> MHHHHHHAAGIPMNNPAIKRIGNHITKSPEDKREYRGLELANGIKVLLISDPTTDKSSAALDVHIGSLSDPPNIAGLSHFLQHMLFLGTKKYPKENEYSQFLSEHAGSSNAFTSGEHTNYYFDVSHEHLEGALDRFAQFFLSPLFDESAKDREVNAVDSEHEKNVMNDAWRLFQLEKATGNPKHPFSKFGTGNKYTLETRPNQEGIDVRQE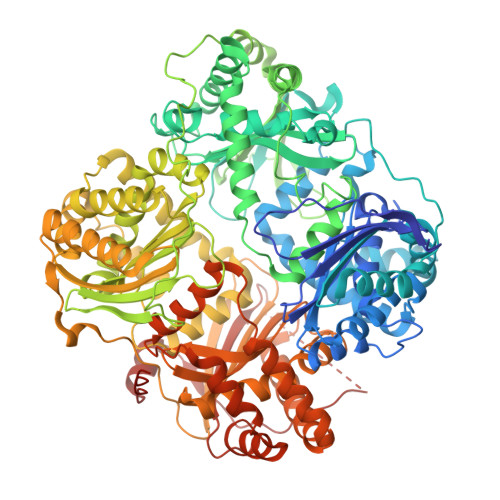LLKFHSAYYSSNLMAVVVLGRESLDDLTNLVVKLFSEVENKNVPLPEFPEHPFQEEHLKQLYKIVPIKDIRNLYVTFPIPDLQKYYKSNPGHYLGHLIGHEGPGSLLSELKSKGWVNTLVGGQKEGARGFMFFIINVDLTEEGLLHVEDIILHMFQYIQKLRAEGPQEWVFQELKDLNAVAFRFKDKERPRGYTSKIAGILHYYPLEEVLTAEYLLEEFRPDLIEMVLDKLRPENVRVAIVSKSFEGKTDRTEEWYGTQYKQEAIPDEVIKKWQNADLNGKFKLPTKNEFIPTNFEILPLEKEATPYPALIKDTAMSKLWFKQDDKFFLPKANLNFEFFSPFAYVDPLHSNMAYLYLELLKDSLNEYAYAAELAGLSYDLQNTIYGMYLSVKGYNDKQPILLKKIIEKMATFEIDEKRFEIIKEAYMRSLNNFRAEQPHQHAMYYLRLLMTEVAWTKDELKEALDDVTLPRLKAFIPQLLSRLHIEALLHGNITKQAALGIMQMVEDTLIEHAHTKPLLPSQLVRYREVQLPDRGWFVYQQRNEVHNNSGIEIYYQTDMQSTSENMFLELFAQIISEPAFNTLRTKEQLGYIVFSGPRRANGIQGLRFIIQSEKPPHYLESRVEAFLITMEKSIEDMTEEAFQKHIQALAIRRLDKPKKLSAESAKYWGEIISQQYNFDRDNTEVAYLKTLTKEDIIKFYKEMLAVDAPRRHKVSVHVLAREMDSNPVVGEFPAQNDINLSQAPALPQPEVIQNMTEFKRGLPLFPLVKPHINFMAAKL>[2x]DQIRYSIPEELAKNSIVGNLARDLGLSVQNLPTRKLRVSAEKDYFTVNPESGDLLVGDRIDREQVCGKQPQCVLEFDIVAEKPLNIFHVAVILQ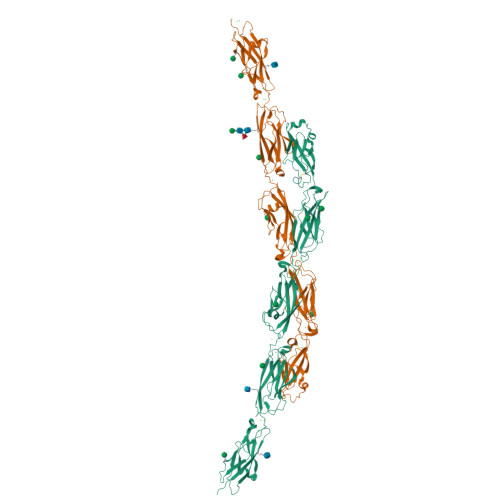DVNDNAPLFKQSEVDLNIGESTRPGKAFPLDPALDLDAGSNSLQKYYLTDNEYFEVTEKETPDGRKYPELILKRFLDREEHNFHQLVLTAVDGGDPPRSGTTQIRIQVTDINDNPPMFSQDVFSVTLREDVPPGFSVLQVTATDQDEGVNAEITYAFHNVDEQVERIFNLDKRTGEITTKDNLDFETAKSYTLNVEAKDPGDLASHCSIQVKILDENDCVPEVIVTSVFTPLPEDSPLGTVIALIKTRDRDSGENGDVYCHVLGNEGFVLKSSSKNYYKLVTDRTLDREAIPEYNVTIVAADRGKPPLSSNVIITLHISDVNDNAPVFHQASYLVHVAENNPPGTSIAQVSASDPDLGSNGLISYSIIASDLEPRALSSFVSVNQDSGVVFAQRAFDHEQLRSFQLTLQARDHGSPTLSANVSMRVLVGDRNDHHHHHHHH> MEKLMFHPHGKEFHHNPFSVLGRFREEEPIHRFELKRFGATYPAWLITRYDDCMAFLKDNRITRDVKNVMNQEQIKMLNVSEDIDFVSDHMLAKDTPDHTRLRSLVHQAFTPRTIENLRGSIEQIAEQLLDEMEKENKADIMKSFASPLPFIVISELMGIPKEDRSQFQIWTNAMVDTSEGNRELTNQALREFKDYIAKLIHDRRIKPKDDLISKLVHAEENGSKLSEKELYSMLFLLVVAGLETTVNLLGSGTLALLQHKKECEKLKQQPEMIATAVEELLRYTSPVVMMANRWAIEDFTYKGHSIKRGDMIFIGIGSANRDPNFFENPEILNINRSPNRHISFGFGIHFCLGAPLARLEGHIAFKALLKRFPDIELAVAPDDIQWRKNVFLRG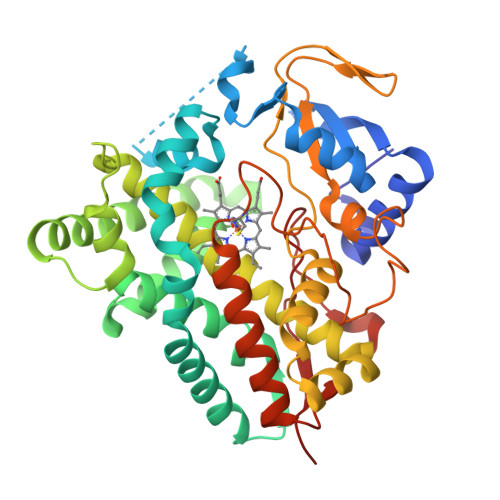LESLPVSLSK>MFKHIIARTPARSLVDGLTSSHLGKPDYAKALEQHNAYIRALQTCDVDITLLPPDERFPDSVFVEDPVLCTSRCAIITRPGAESRRGETEIIEETVQRFYPGKVERIEAPGTVEAGDIMMVGDHFYIGESARTNAEGARQMIAILEKHGLSGSVVRLEKVLGLKTGLAYLEHNNLLAAGEFVSKPEFQ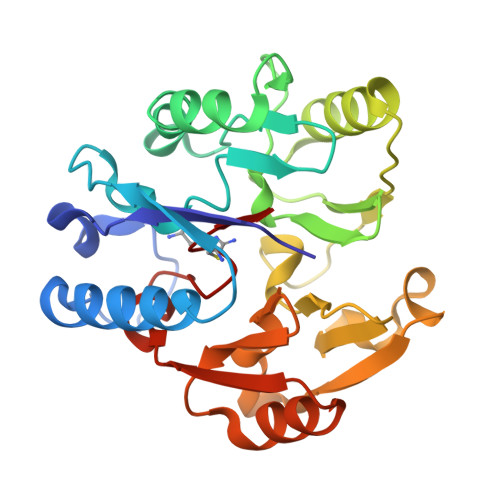DFNIIEIPEEESYAANCIWVNERVIMPAGYPRTREKIARLGYRVIEVDTSEYRKIDGGVSCMSLRF[2x]>[4x]MKGPFTEAEDDLIREYVKENGP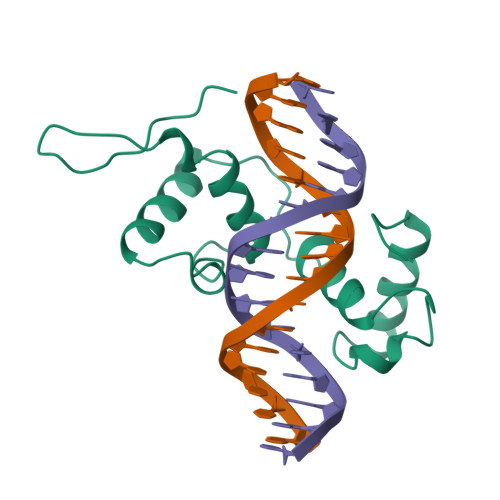QNWPRITSFLPNRSPKQCRERWFNHLDPAVVKHAWTPEEDETIFRNYLKLGSKWSVIAKLIPGRTDNAIKNRWNSSISKRISTNSNHKEILLPDRSKKRKAADVPKKLE In most bacteria, iron homeostasis is regulated primarily by the ferric uptake regulator (Fur). Fur, which was first discovered in Escherichia coli, is a global transcriptional regulator that directly controls the transcription of over 90 genes involved in iron uptake, storage and metabolism. Several holo-Fur structures have been solved, revealing a modular domain organization including an N-terminal DNA-binding domain (DBD) and a C-terminal dimerization domain (DD). In this study, we present six crystal structures of apo-Fur, holo-Fur, Fur in complex with the Fe2+ transport protein (feoAB1) operator and the P. aeruginosa (or E. coli) Fur box.

The apo-MgFur structure was determined at 1.55 Å resolution. The results showed that apo-Fur is made of two monomers that form a stable dimer, with both monomers consisting of residues 1–134 and nine disordered C-terminal residues. Each monomer exhibited a modular architecture, including an N-terminal DBD and C-terminal DD, connected by a flexible hinge formed by residues 83–88. The dimeric interface was primarily formed by the DD, which was composed of two α5 and two β5 that formed intermolecular hydrophobic interactions and an antiparallel β-sheet, respectively. The buried interface comprised 1,628.4 Å2 per molecule, indicating a very strong interaction between the monomers. Overall conformations of the two Fur monomers, especially in the hinge region, differed greatly, with an overall root mean squared deviation (r.m.s.d.) of 4.6 Å. However, their DD and DBD conformations were almost identical (r.m.s.d.=0.9 and 0.4 Å, respectively). Analysis of the crystal packing of the apo-Fur structure revealed that the DBD is stabilized by other DBDs and DDs from symmetric units. No absorption peak of transition metal ions was found by X-ray absorption spectroscopy, suggesting that the metal ion-binding sites are not occupied in apo-Fur. In this study, we solved the first apo-Fur structure without transition metal ions and found that apo-MgFur is a transition metal ion-independent dimer, providing a structural basis for further studies of apo-Fur.

>GHMVSRIEQRCIDKGMKMTDQRRVIAQVLSDSADHPDVEEVYRRATAKDPRISIATVYRTVRLFEEESILERHDFGDGRARYEEAPSEHHDHLIDVNSARVIEFTSPEIEALQREIARKHGFRLVGHRLELYGVPLTSGGDSDDK[2x]>MGSMHVTLVEINVHEDKVDEFIEVFRQNHLGSVQEEGNLRFDVLQDPEVNSRFYIYEAYKDED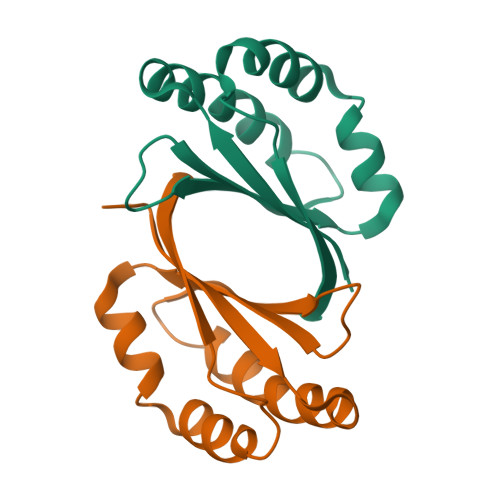AVAFHKTTPHYKTCVAKLESLMTGPRKKRLFNGLMP[4x]> ERH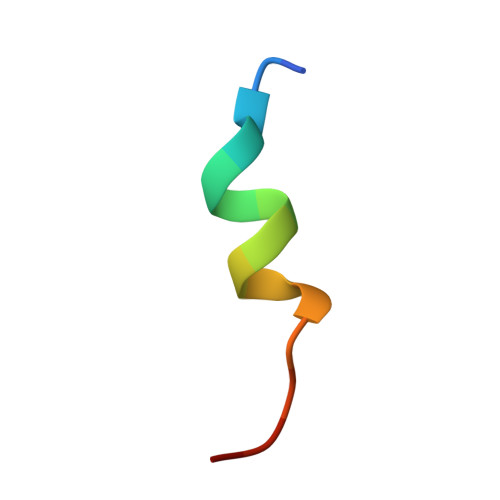KILHRLLQEGSPS> MELLTFKNGVHPPHGKHYTENKPIEEYLPKGDIVIPMSQHIGAPAEPIVKKGDRVLVGQKIGEAKGFVSANIHASVS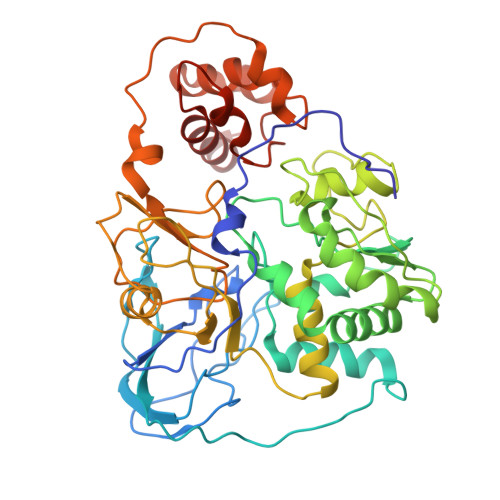GTVKNVAPVTLFNGVKSTAVIIENDGQYEEIETEKRDYTKLSNEEIINIIKEAGIVGMGGATFPTHVKLAPPPDKNIDSIVVNAAECEPYLTCDHRMMLEKTNEIVEGLKIVLKLFPKATGYIGIEDNKMNAIKAMQEAVKNIANIEVKAVKTKYPQGAEKQLIYAITKREVPSGGLPADAGCIVQNVDTIYEIYNAVVNGKPLTSRVVTVTGDAIKEPKNLRFKIGTSVRELVEAAGGFAEEPLKVISGGPMMGMAMYSLDVPSTKGTSGVLCLTKKVAEIEEESNCINCGKCVQVCPMNLMPTKLATASAVSNLDMFNEFSGRDCIECGCCSFVCPARRHLLQRIRSGKKAVSKKK>[6x]MSKDYQSLAKLSPFELKDELIKIASSDGNRLMLNAGRGNPNFLATTPRRAFFRLGLFAAAESELSYSYMTTVGVGGLAKIDGIEGRFERYIAENRDQEGVRFLGKSLSYVRDQLGLDPAAFLHEMVDGILGCNYPVPPRMLNISEKIVRQYIIREMGADAIPSESVNLFAVEGGTAAMAYIFESLKLNGLLKAGDKVAIGMPVFTPYIEIPELAQYALEEVAINADPSLNWQYPDSELDKLKDPAIKIFFCVNPSNPPSVKMDQRSLERVRNIVAEHRPDLMILTDDVYGTFADDFQSLFAICPENTLLVYSFSKYFGATGWRLGVVAAHQQNVFDLALDKLQESEKVALDHRYRSLLPDVRSLKFIDRLVADSRAVALNHTAGLSTPQQVQMALFSLFALMDEADEYKHTLKQLIRRRETTLYRELGMPPLRDENAVDYYTLIDLQDVT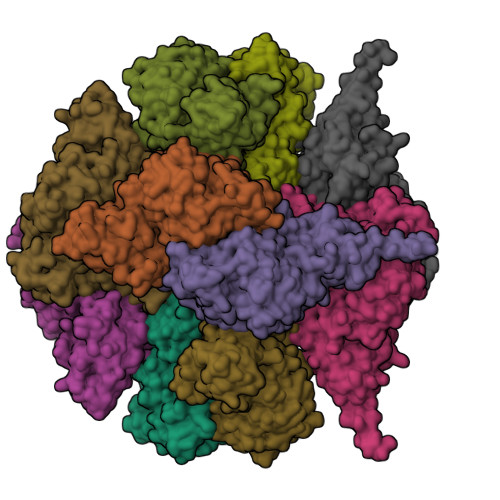AKLYGEAFSEWAVKQSSTGDMLFRIADETGIVLLPGRGFGSNRPSGRASLANLNEYEYAAIGRALRKMADELYAEYSGQAQNLKLAAALEHHHHHH>[2x]MADSELQLVEQRIRSFPDFPTPGVVFRDISPVLKDPASFRAAIGLLARHLKATHGGRIDYIAGLDSRGFLFGPSLAQELGLGC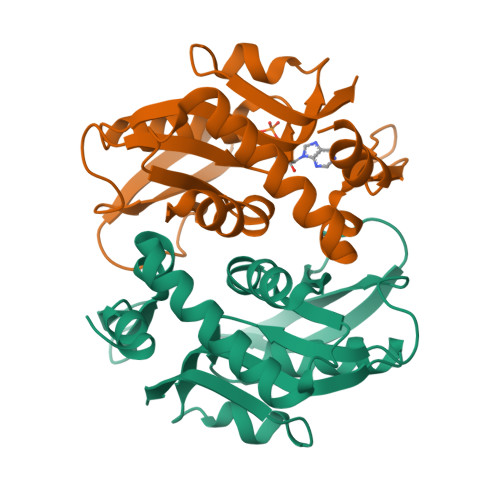VLIRKRGKLPGPTLWASYSLEYGKAELEIQKDALEPGQRVVVVDDLLATGGTMNAACELLGRLQAEVLECVSLVELTSLKGREKLAPVPGFSLLQYE> FSCNVDGG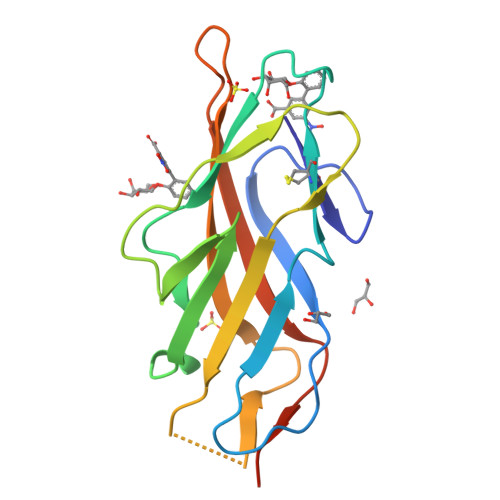SSIGAGTTSVYVNLDPVIQPGQNLVVDLSQHISCWNDYGGWYDTDHINLVQGSAFAGSLQSYKGSLYWNNVTYPFPLTTNTNVLDIGDKTPMPLPLKLYITPVGAAGGVVIKAGEVIARIHMYKIATLGSGNPRNFTWNIISNNSVVMPTGGHHHHHH> MTSEQTGEPAEDTSGVIKMAVKADRRAYPAQITPKMCLLEWCRREKLAQPVYETVQRPLDRLFSSIVTVAEQKYQSTLWDKSKK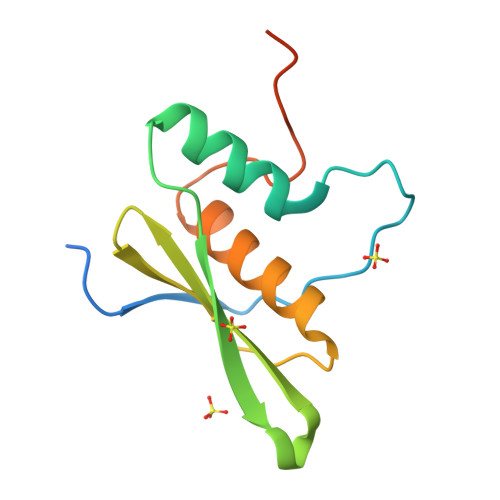LAEQAAAIVCLRSQGLPEGRLGEESPSLHKHHHHHH>[5x]SPVEWTVMDVVEYFTEAGFPEQATAFQEQEIDGKSLLLMQRTDVLTGLSIRL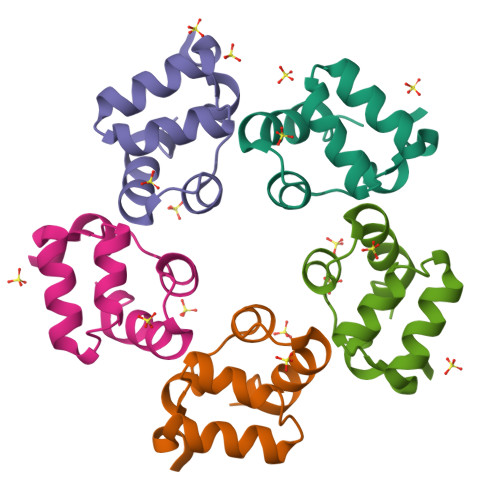GPALKIYEHHIKVL> MKFKWDEFFVTGDPLILGAQVSIALSTIAIIFVLTYFKKWKWLWSEWITTVDHKKLGIMYIISAVIMLFRGGVDGLMMRAQLALPNNSFLDSNHYNEIFTTHGTIMIIFMAMPFLIGLINVVVPLQIGARDVAFPYLNNLSFWTFFVGAMLFNISFVIGGSPNAGWTSYMPLASNDMSPGPGENYYLLGLQIAGIGTLMTGINFMVTILKMRTKGMTLMRMPMFTWTTLITMVIIVFAFPVLTVALALLSFDRLFGAHFFTLEAGGMPMLWANLFWIWGHPEVYIVILPAFGIFSEIISSFARKQLFGYKAMVGSIIAISVLSFLVWTHHFFTMGNSASVNSFFSITTMAISIPTGVKIFNWLFTMYKGRISFTTPMLWALAFIPNFVIGGVTGVMLAMAAADYQYHNTYFLVSHFHYVLIAGTVFACFAGFIFWYPKMFGHKLNERIGKWFFWI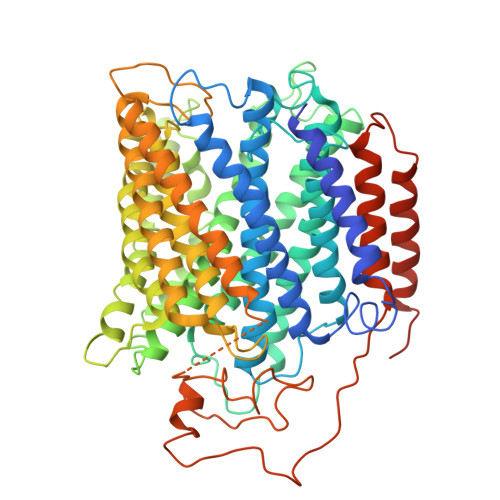FMIGFNICFFPQYFLGLQGMPRRIYTYGPNDGWTTLNFISTVGAFMMGVGFLILCYNIYYSFRYSTREISGDSWGVGRTLDWATSSAIPPHYNFAVLPEVKSQDAFLHMKEEKTELYPESKFKKIHMPSNSGRPFFMSVAFGLAGFGLVFEWYWMGVVGLIGVLLCMVLRSFEYDNGYYISVDEIKETERKISE>GSIGQEMQMGDYYVRQLRGSAPLINDPLLTQYINSLGMRLVSHANSVKTPFHFFLINNDEINAFAFFGGNVVLHSALFRYSDNESQLASVMAHEISHVTQRHLARAMEDQQRSAPLTWVGALGSILLAMASPQAGMAALTGTLAGTRQGMISFTQQNEQEADRIGIQVLQRSGFDPQAMPTFLEKLLDQARYSSRPPEILLTHPLPESRLADARNRANQMRPMVVQSSEDFYLAKARTLGMYNSGRNQLTSDLLDEWAKGNVRQQRAAQYGRALQAMEANKYDEARKTLQPLLAAEPGNAWYLDLATDIDLGQNKANEAINRLKNARDLRTNPVLQLNLANAYLQGGQPQEAANILNRYTFNNKDDSNGWDLLAQAEAALNNRDQELAARAEGYALAGRLDQAISLLSSASSQVKLGSLQQA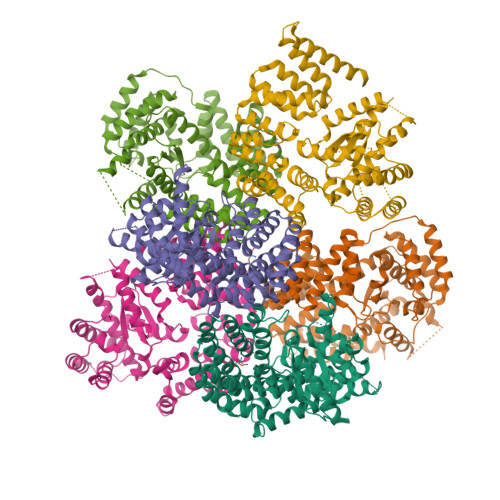RYDARIDQLRQLQERFK[6x]>[2x]MSQAATPAADGKVKISIDPLTRVEGHLKIEVEVKDGKVVDAKCSGGMFRGFEQILRGRDPRDSSQIVQRICGVCPTAHCTASVMAQDDAFGVKVTTNGRITRNLIFGANYLQSHILHFYHLAALDYVKGPDVSPFVPRYANADLLTDRIKDGAKA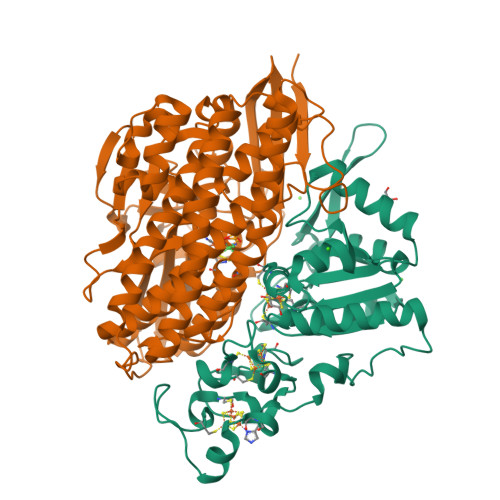DATNTYGLNQYLKALEIRRICHEMVAMFGGRMPHVQGMVVGGATEIPTADKVAEYAARFKEVQKFVIEEYLPLIYTLGSVYTDLFETGIGWKNVIAFGVFPEDDDYKTFLLKPGVYIDGKDEEFDSKLVKEYVGHSFFDHSAPGGLHYSVGETNPNPDKPGAYSFVKAPRYKDKPCEVGPLARMWVQNPELSPVGQKLLKELYGIEAKNFRDLGDKAFSIMGRHVARAEETWLTAVAVEKWLKQVQPGAETYVKSEIPDAAEGTGFTEAPRGALLHYLKIKDKKIENYQIVSATLWNANPRDDMGQRGPIEEALIGVPVPDIKNPVNVGRLVRSYDPULGCAVH;>[2x]MTEGAKKAPVIWVQGQGCTGCSVSLLNAVHPRIKEILLDVISLEFHPTVMASEGEMALAHMYEIAEKFNGNFFLLVEGAIPTAKEGRYCIVGETLDAKGHHHEVTMMELIRDLAPKSLATVAVGTCSAYGGIPAAEGNVTGSKSVRDFFADEKIEKLLVNVPGCPPHPDWMVGTLVAAWSHVLNPTEHPLPELDDDGRPLLFFGDNIHENCPYLDKYDNSEFAETFTKPGCKAELGCKGPSTYADCAKRRWNNGINWCVENAVCIGCVEPDFPDGKSPFYVAE> TLVHVASVEKGRSYEDFQKVYNAIALKLREDDEYD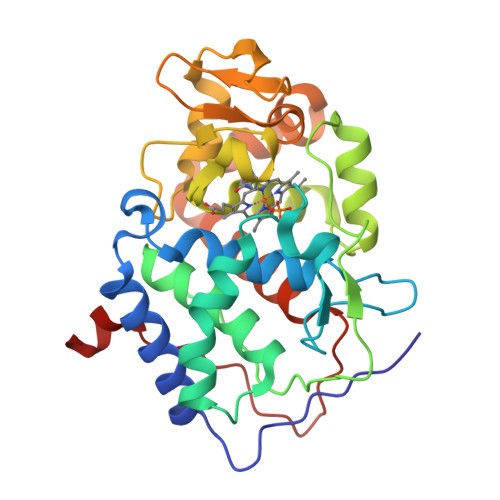NYIGYGPVLVRLAWHISGTWDKHDNTGGSYGGTYRFKKQFNDPSNAGLQNGFKFLEPIHKEFPWISSGDLFSLGGVTAVQEMQGPKIPWRCGRVDTPEDTTPDNGRLPDADKDAGYVRTFFQRLNMNDREVVALMGAGALGKTHLKNSGYEGPWGAANNVFTNEFYLNLLNEDWKLEKNDANNEQWDSKSGYMMLPTDYSLIQDPKYLSIVKEYANDQDKFFKDFSKAFEKLLENGITFPKDAPSPFIFKTLEEQGL>ETGTVPAINYLGAGYDHVRGNPVGDPSSMGDPGIRPPVLRFTYAQNEDGVSNDLTVLQPLGGYVRQYVACRQSETISELSNLSDYQNELSVDASLQGGDPIGLNSFSASTGYRDFAKEVSKKDTRTYMLKNYCMRYEAGVAQSNHFKWNVTLAFAAGVSQLPDVFDAHNPECACSAEQWRQDQNAEACTKTNVPIWISFIEQFGTHFLVRLFAGGKMTYQVTAKRSEVEKMRNMGIDVKTQLKMQLGGVSGGAGQGTSSKKQ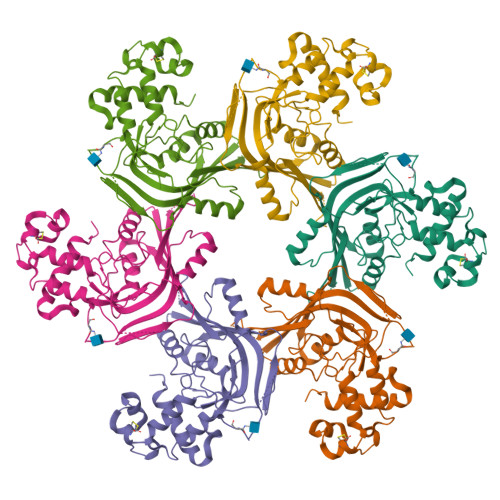QSSSEYQMNVQKETLVIGGRPPGQVSDPAALAAWADTVEELPMPVKFEVQPLYHLLPVEKQEAFKQAVTFYSKAVGLTPQDLSALGTKHHHHHH[6x]>MKLLKDLLVDRKEFEDWKNNLTWARDGTLYLTTFPDISIGQPKYAKDINCNSKNLFHVKEFPLEFENKLDFELAQQNGLLNSQPVCYPRVCKPSPIDDWMAVLSNNGNVSVFKDNKMLTNLDSKGNLSSRTYHCFEWNPIESSIVVGNEDGELQFFSIRKNSENTPEFYFESSIRLSDAGSKDWVTHIVWYEDVLVAALSNNSVFSMTVSASSHQPVSRMIQNASRRKITDLKIVDYKVVLTCPGYVHKIDLKNYSISSLKTGSLENFHIIPLNHEKESTILLMSNKTSYKVLLEDELHVTADNIIAPYLEKKFKKWSTIWNEFNNYETTLVIHGISLSPDGYSIAIVYDMERVAFKYKIASEQSFNIMFAPLYHTWTISERAVGLAWYQTYQIYNQSLPKLPENFSMNKKLLNGNYPISLDFQSYLNALMKSEEMRIIMFLNMTIDKPSILSFLEALYEYAINKKSELTNSFDLACVLSIAAILKREAPIYNGTLLMKNSFLEETFNLESFTADPETVTSTTNNTWKRCGVTLLPILTTHVKICPVSKQRVIDIKRDDLNDYGWFTRGLLERFNEISVYCGTTLEVM[2x];>MGLLKDLSSARDKIERIYGLNKEKLLLLAKVKEGFETSVFDFPFKNIQPDSPYFVCLDPPCKKESAYNKVIGDKNRTVYHEINKTEFENMIKLRTKRLKLLIGEVDAEVSTGDKIEFPVLANGKRRGFIYNVGGLVTDIAWLNIEENTDIGKDIQYLAVAVSQYMDEPLNEHLEMFDKEKHSSCIQIFKMNTSTLHCVKVQTIVHSFGEVWDLKWHEGCHAPHLVGCLSFVSQEGTINFLEIIDNATDVHVFKMCEKPSLTLSLADSLITTFDFLSPTTVVCGFKNGFVAEFDLTDPEVPSFYDQVHDSYILSVSTAYSDFEDTVVSTVAVDGYFYIFNPKDIATTKTTVSRFRGSNLVPVVYCPQIYSYIYSDGASSLRAVPSRAAFAVHPLVSRETTITAIGVSRLHPMVLAGSADGSLIITNAARRLLHGIKNSSATQKSLRLWKWDYSIKDDKYRIDSSYEVYPLTVNDVSKAKIDAHGINITCTKWNETSAGGKCYAFSNSAG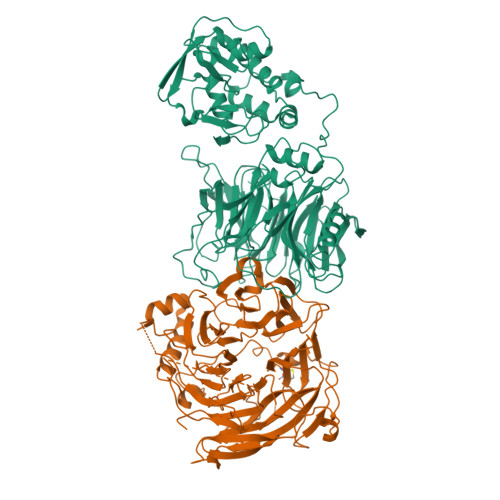LLTLEYLSLEHHHHHH[2x]>[2x]MGSDKIHHHHHHMQVRIERAERIESELEEHVGDQTFVEESRFLEEDEQREGEILDQIIFVDGKRRSFVRITTDEGITGIFAELCVGAVIWDREGGTKTLFSPDKPPVKERVLGFSQSFQEEGYEEVGGILFKVVKEGKDAMQSIDLYMRSLEIEEVRKHMDKNILIVKDGPAARELPFE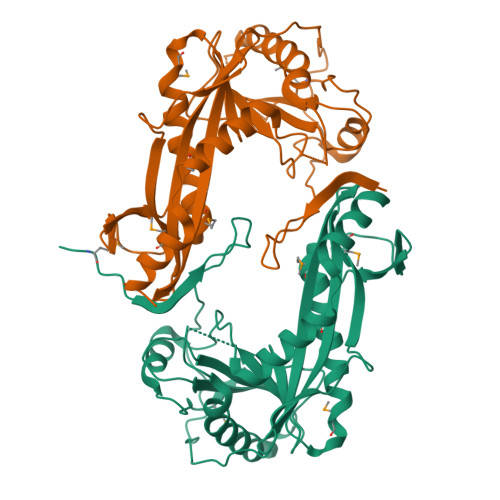ENVGPIGLVKNIGVTELSKEDFKKLRFLKKGKRSKMFVSSRETPLKKVGAYVKLIDGEGIRGLVRLETYVKDDNQIPYIRKVFDDLAKTLPHLTADLPIPRLPENILPIQFLEENLSYYLTDKNYMNTRLFAYIGR> SAHTESVCVHAGTATGADLHWLNAICTGKSTYTVNCAPAGNKNAGSTHTGTCPAGQDCFQLEQVGNFWGDREPDATCSP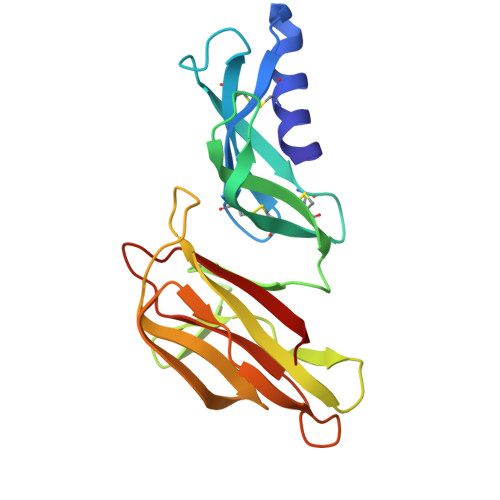SNTVFDAVDDKEATHVNGKVVTRAGKPGIGRKLIRLKAQVYRRDGHYGQTSRMGFFRNGKEVYHIDNVASMEPTWNFDPSSDQSFSFFFTPGPNAFRIQGTLNLAS> HHHHHHAQLPSPTNGKKWEKVEQLSDEFNGNSIDTNKWYDYHPFWEGRAPSNFKKGNAFVSDGFLNLRSTLRKEPSSVQDPFKDIWVDAAAAVSKTKAQPGYYYEARFKASSLSMTSSFWFRVGQFSEIDVIEHIGNPSKENRQDDLP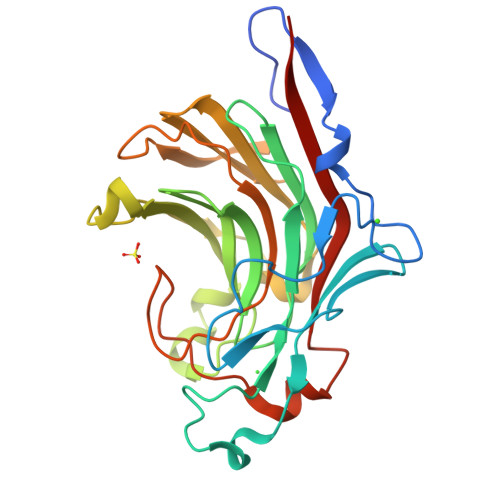YQYHVNTHYYGKHAGLQPLGTEYKMPGRGRDNFYTYGFWWKSPNELLFYFNGKQVMRIVPRVPLDEELRMIFDTEVFPFATAGVANIGLPKPENLRDNSKNTMKVDWVRVYKLVDGTA> MRAEGLGGLERFCSPGKGRGLRALQPFQVGDLLFSCPAYAYVLTVNERGNHCEYCFTRKEGLSKCGRCKQAFYCNVECQKEDWPM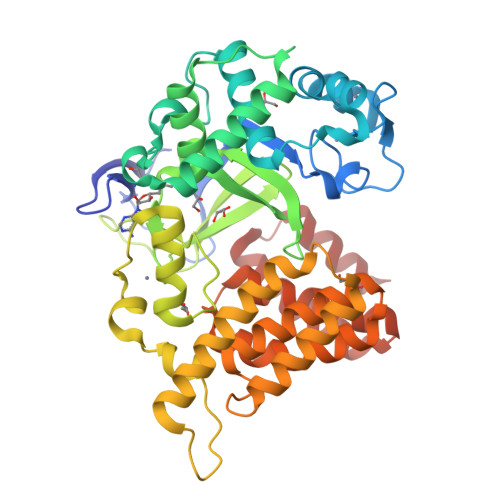HKLECSPMVVFGENWNPSETVRLTARILAKQKIHPERTPSEKLLAVKEFESHLDKLDNEKKDLIQSDIAALHHFYSKHLGFPDNDSLVVLFAQVNCNGFTIEDEELSHLGSAIFPDVALMNHSCCPNVIVTYKGTLAEVRAVQEIKPGEEVFTSYIDLLYPTEDRNDRLRDSYFFTCECQECTTKDKDKAKVEIRKLSDPPKAEAIRDMVRYARNVIEEFRRAKHYKSPSELLEICELSQEKMSSVFEDSNVYMLHMMYQAMGVCLYMQDWEGALQYGQKIIKPYSKHYPLYSLNVASMWLKLGRLYMGLEHKAAGEKALKKAIAIMEVAHGKDHPYISEIKQEIESH(1R,2R)-2,4,4-trimethyl-N-[(1H-pyrazol-3-yl)methyl]cyclopentan-1-amine | C12 H21 N3 | 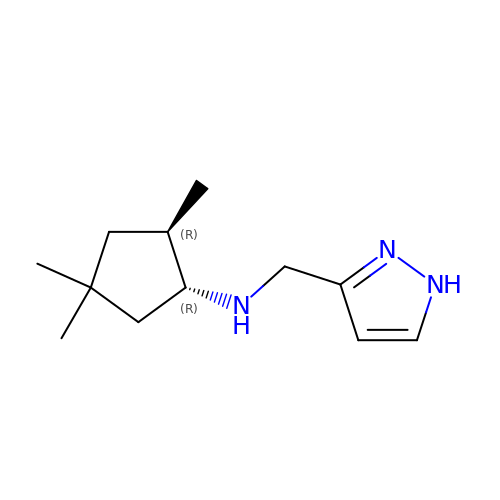VJSXSAJVDGYBFZ-MWLCHTKSSA-N>MIHLYDAKSFAKLRAAQYAAFHTDAPGSWFDHTSGVLESVEDGTPVLAIGVESGDAIVFDKNAQRIVAYKEKSVKAEDGSVSVVQVENGFMKQGHRGWLVDLTGELVGCSPVVAEFGGHRYASGMVIVTGKGNSGKTPLVHALGEALGGKDKYATVRFGEPLSGYNTDFNVFVDDIARAMLQHRVIVIDSLKNVIGAAGGNTTSGGISRGAFDLLSDIGAMAASRGCVVIASLNPTSNDDKIVELVKEASRSNSTSLVISTDVDGEWQVLTRTGEGLQRLTHTLQTSYGEHSVLTIHTSKQSGGKQASGKAIQTVIKNDELESVLRRLTSN[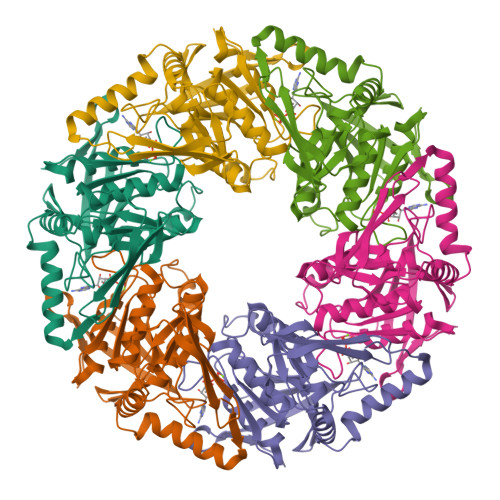3x]> MPLNRTLEMSELPGLEDWEDEFDLENAVLFEVAWEVANKVGGIYTVLQTKAKVTGDEWGDNYFLVGPYTEQGVRTQVELLEAPTPALKRTLDSMNSKGCK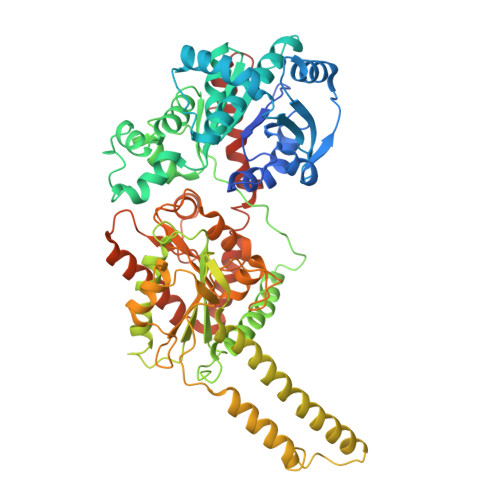VYFGRWLIEGGPLVVLLDVGASAWALERWKGELWDTCNIGVPWYDREANDAVLFGFLTTWFLGEFLAQSEEKPHVVAHFHEWLAGVGLCLCRARRLPVATIFTTHATLLGRYLCAGAVDFYNNLENFNVDKEAGERQIYHRYCMERAAAHCAHVFTTVSQITAIEAQHLLKRKPDIVTPNGLNVKKFSAMHEFQNLHAQSKARIQEFVRGHFYGHLDFNLDKTLYFFIAGRYEFSNKGADVFLEALARLNYLLRVNGSEQTVVAFFIMPARTNNFNVETLKGQAVRKQLWDTANTVKEKFGRKLYESLLVGSLPDMNKMLDKEDFTMMKRAIFATQRQSFPPVCTHNMLDDSSDPILTTIRRIGLFNSSADRVKVIFHPEFLSSTSPLLPVDYEEFVRGCHLGVFPSYYEPWGYTPAECTVMGIPSISTNLSGFGCFMEEHIADPSAYGIYILDRRFRSLDDSCSQLTSFLYSFCQQSRRQRIIQRNRTERLSDLLDWKYLGRYYMSARHMALSKAFPEHFTYEPNEADAAQGY Carbapenemases are the main cause of carbapenem resistance in Gram‐negative bacteria. How β‐lactamases with weak carbapenemase activity, such as the OXA‐10‐type class D β‐lactamases, contribute to anti‐bacterial drug resistance is unclear. OXA‐655 is a T26M and V117L OXA‐10 variant, recently identified from hospital wastewater. Here, we have solved crystal structures of OXA‐10 in complex with imipenem (IPM) and ETP, and OXA‐655 in complex with MEM in order to unravel the structure–function relationship and the impact of residue 117 in enzyme catalysis.

Despite exhibiting stronger carbapenemase activity towards ertapenem (ETP) and meropenem (MEM) in Escherichia coli, OXA‐655 exhibits reduced activity towards oxyimino‐substituted β‐lactams like ceftazidime. The new crystal structures show that L117 is situated at a critical position with enhanced Van der Waals interactions to L155 in the omega loop. This restricts the movements of L155 and could explain the reduced ability for OXA‐655 to bind a bulky oxyimino group. The V117L replacement in OXA‐655 makes the active site S67 and the carboxylated K70 more water exposed. This could affect the supply of new deacylation water molecules required for hydrolysis and possibly the carboxylation rate of K70. But most importantly, L117 leaves more space for binding of the hydroxyethyl group in carbapenems.

>MKTFAAYVIIACLSSTALAGSITENMSWNKEFSAEAVNGVFVLCKSSSKSCATNDLARASKEYLPASTFKIPNAIIGLETGVIKNEHQVFKWDGKPRAMKQWERDLTLRGAIQVSALPVFQQIAREVGEVRMQKYLKKFSYGNQNISGGIDKFWLEGQLRISAVNQVEFLESLYLNKLSASKENQLIVKEALVTEAAPEYLVHSKTGFSGVGTESNPGVAWWVGWVEKETEVYFFAFNMDIDNESKLPLRKSIPTKIMESEGIIGG[4x]> GPVEESVERAMVRVADTVSSKPTNSESIPALTAAETGHTSQVVPSDTMQTRHVKNYHSRSESSIENFLCRSACVYYATYNNNSEKGYAEWVINTRQVAQLLRRKLEFTYLRFDLELTFVITSAQEPSTATSVDAPVQTQQIMYVPPGGPVPTKVTDYAWQTSTNPSVFWTEGNAPPRMSIPFISIGNAYSCFYDGWTQFSRNGVYGINTLNNMGTLYMRHVNEAGQGPIKSTVRIYFKPKHVKAWVPRPPRLCQYEKQKNVNFNPTGVTTTRSNITTT;> SPSAEECGYSDRVRSITLGNSTITTQECANVVVGYGVWPEYLKDNEATGEDQPTQPDVATCRFYTLESVQWMKNSAGWWWKLPDALSQMGLFGQNMQYHYLGRTGYTIHVQCNASKFHQGCLLVVCVPEAEMGCSNLNNTPKFAELSGGDNARMFTDTEVGTSNDKKVQTAVWNAGMGVGVGNLTIFPHQWINLRTNNSATIVMPYINSVPMDNMYRHNNLTLMIIPFVPLNYSEGSSPYVPITVTIAPMCAEYNGLRLASSQ;> GLPVMTTPGSTQFLTSDDFQSPSAMPQFDVTPEMQIPGRVNNLMEIAEVDSVVPVNNTDNNVNGLKAYQIPVQSNSDNRRQVFGFPLQPGANNVLNRTLLGEILNYYTHWSGSIKLTFMFCGSAMATGKFLLAYSPPGAGVPKNRRDAMLGTHVIWDVGLQSSCVLCVPWISQTHYRYVVEDEYTAAGYVTCWYQTNIIVPADVQSTCDILCFVSACNDFSVRMLKDTPFIRQDNFYQ;> GAQVSTQKTGAHETGLNASGNSIIHYTNINYYKDAASNSANRQDFTQDPGKFTEPVKDIMIKSMPALN

The genus Enterovirus within the Picornaviridae, a family of non-enveloped viruses with a positive single-stranded RNA genome, is comprised of more than 100 serotypes. Human enteroviruses (EV) are presently classified into four groups, Enterovirus A-D (EV-A, B, C, and D), among which EV-B, the largest group, consists of over 60 serotypes, including all 6 serotypes of coxsackievirus B (CVB1-6), coxsackievirus A9 (CVA9), over 30 serotypes of echoviruses and more than 20 newly identified enteroviruses. The capsid proteins (VP1, VP2, and VP3) adopt the classical eight-stranded anti-parallel β-barrel configuration with the N-termini residing inside and the C-termini exposed on the surface. Most of the uncoating receptors bind to the “canyon” sites of the viral particle, dislodging the “pocket factor” in VP1 and subsequently triggering conformational changes of the intact particle to release the genome, albeit that SCARB2 binds EV71 outside the canyon.

Given that three key structural elements of the VP1 GH, VP2 EF, and VP1 EF loops dominate virus–receptor interactions, we systematically calculated pairwise Euclidean distances between all amino acids for all possible (n2) pairs of these three key elements from 15 structure-available human EVs, which defines a k (k = (n2)) dimensional space delineating the structural characteristics of the receptor-recognition sites. The phylogenetic tree could clearly separate these human EVs into three groups: EV-A, EV-B, and EV-C. Within each group, viruses with distinct receptors were further grouped into mono-phylogenetic clades. This structure-based in silico analysis completely matches the results of experimentally derived receptor identification, therefore, it can be used to deduce the receptor usage for human EVs. To test the robustness of our structure-based algorithm, we determined the structures of three other human EVs (CVB1, CVB5 and Echovirus 3) and put these into our algorithm. The in silico analysis suggests that CVB1 and CVB5 are CAR-dependent human EVs and E3 utilizes FcRn as a functional receptor, predictions consistent with experimental reports.> MAVLGLQGVRGGVGTTTITAALAWSLQMLGENVLVVDACPDNLLRLSFNVDFTHRQGWARAMLDGQDWRDAGLRYTSQLDLLPFGQLSIEEQENPQHWQTRLSDICSGLQQ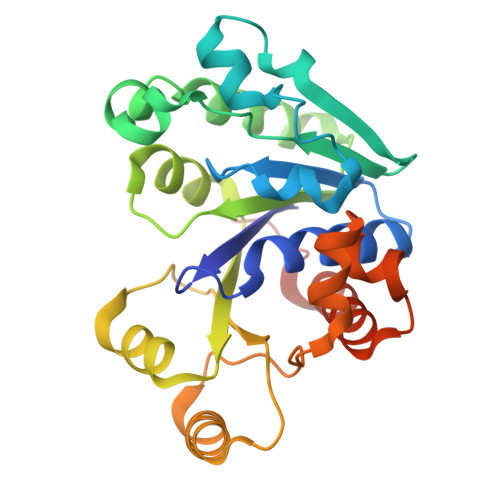LKASGRYQWILIDLPRDASQITHQLLSLCDHSLAIVNVDANCHIELHQQALPDGAHILINNFRIGSQVQDDIYQLWLQSQRRLLPMLIHRDEAMAECLAAKQPVGEYRSDALAAEEILTLANWCLLNYSGLKTPVGSKS>GASRTERLLNLLLALLNTKVGLPRAVLREKVYHDSADNDVAFGRMFERDKVDLKQFGFEIETLMDPRNFGADDPASARYRIGKDSNRLPDVSLTPAESTVLLLAAQLWERAALGSAAANAVRKLQAAGGFRDVDLPAGVQPRIKPAGQAFDDVVAAMHGKHPIRFGYQAVSTGREEVREVEPWGLGSRFGQWYLVGLDRGRGAKRVFRLSRMTTAISVLTTGSFHPPKDFNARAELDELNELPVRQATLVIDKDKLLALRKKATSLQDAPDESGRDRITVDFRDPEQLAEELASYGPHVKVTGPAELSAAVVRRLQAAADFDDAPLPPLEFPEAGRAPRARKRTSEDQLARMLQLVPFLVHHQGLHIQEVADHFGISRKALIDDLKILICSGLPEGYPDDLLDIQWENDHVYISEHLDLNRPVRFSEEEAAALLTGLAMLGDLPALAGVPEDGSGSALESVTIKLTGAAGEAARLAGSVSGQSVAPEQAQAFAAITQAIREGRQLRLRYFSLQRDEVTERDVDPLRLYSLDSTWYFEAYCHSKAGVRNFRLDRVESLEPNGRAVSGSATAGQDFPAR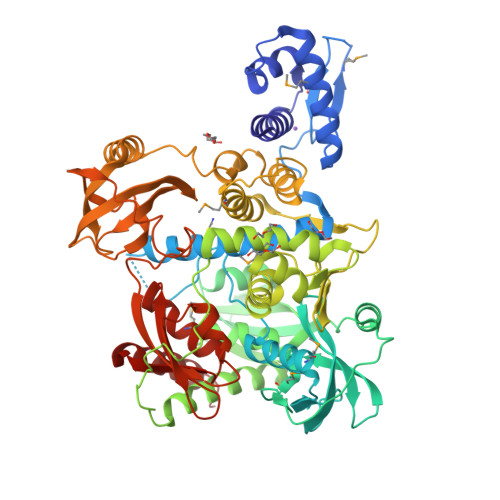LFTPGEDDVLVCLELTRQGAGLADDYYAERTAPLPDGGLLAEVRFGDAGWLPMFVSQHGGSVRILEPESLRQETRAWIDAALVQYDS[2x]> FASLSRFVETLVVADDKMAAFHGAGLKRYLLTVMAAAAKAFKHPSIRNPVSLVVTRLVI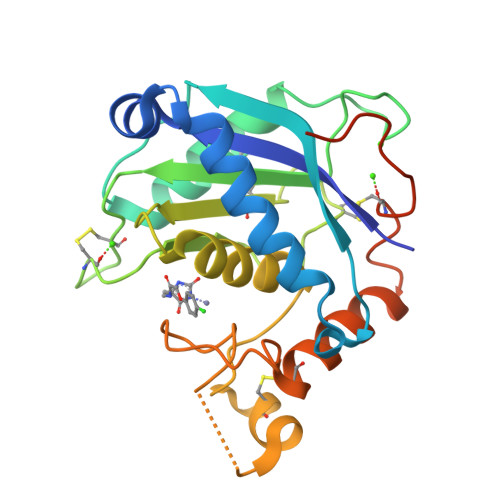LGSGEEGPQVGPSAAQTLRSFCAWQRGLNTPEDSDPDHFDTAILFTRQDLCGVSTCDTLGMADVGTVCDPARSCAIVEDDGLQSAFTAAHELGHVFNMLHDNSKPCISLNGPLSTSRHVMAPVMAHVDPEEPWSPCSARFITDFLDNGYGHCLLDKPEAPLHLPVTFPDVHHHHHH> FQFVTPVGTQNGLKATCAKISPDGQFLAITQGLNILIYDINRRTVSQTLVTSHARPFSELCWSPDGQCIATASDDFSVEIIHLSYGLLHTFIGHTAPVISLTFNRKGNLLFTSSMDESIKIWDTLNGSLMKTISAHS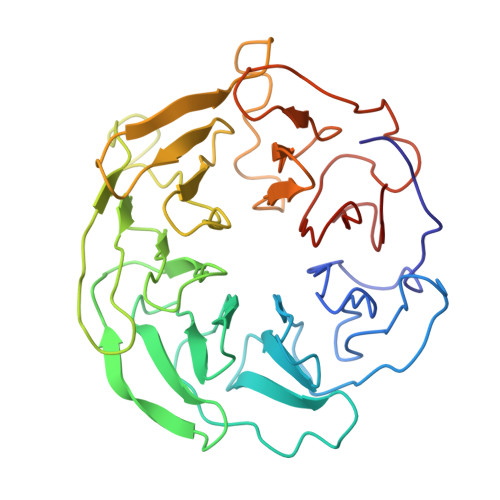EAVVSVDVPMNDSSILSSGSYDGLIRIFDAETGHCLKTLTYDKDWKRENGVVPISQVKFSENARYLLVKSLDGVVKIWDCIGGCVVRTFQVQPLEKGVLHHSCGMDFLNPEDGSTPLVISGYENGDIYCWNSDTKSLLQLLDGSLYHHSSPVMSIHCFGNIMCSLALNGDCCLWRWV N~6~-[5-methyl-4-(1-methylpiperidin-4-yl)-2-(propan-2-yloxy)phenyl]-N~4~-[2-(propan-2-ylsulfonyl)phenyl]-2H-pyrazolo[3,4-d]pyrimidine-4,6-diamine | C30 H39 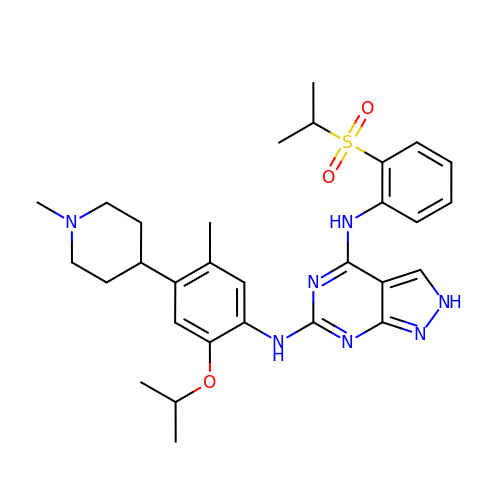N7 O3 S | CWXBESRGEPLREF-UHFFFAOYSA-N> MTHGAVKTYGIRLRVWGDYACFTRPEMKVERVSYDVMPPSAARGILEAIHWKPAIRWIVDRIHVLRPIVFDNVRRNEVSSKIPKPNPATAMRDRKPLYFLVDDGSNRQQRAATLLRNVDYVIEAHFELTDKAGAEDNAGKHLDIFRRRARAGQSFQQPCLGCREFPASFELLEGDVPLSCYAGEKRDLGYMLLDIDFERDMTPLFFKAVMEDDVITPPSRTSPEVRA;>MTAIANRYEFVLLFDVENGNPNGDPDAGNMPRIDPETGHGLVTDVCLKRKIRNHVALTKEGAERFNIYIQEKAILNETHERAYTACDLKPEPKKLPKKVEDAKRVTDWMCTNFYDIRTFGAVMTTEVNCGQVRGPVQMAFARSVEPVVPQEVSITRMAVTTKAEAEKQQGDNRTMGRKHIVPYGLYVAHGFISAPLAEKTGFSDEDLTLFWDALVNMFEHDRSAARGLMSSRKLIVFKHQNRLGNAPAHKLFDLVKVSRAEGSSGPARSFADYAVTVGQAPEGVEVKEML[7x];> MILQALHGYYQRMSADPDAGMPPYGTSMENISFALVLDAKGTLRGIEDLREQEGKKLRPRKMLVPIAEKKGNGIKPNFLWENTSYILGVDAKGKQERTDKCHAAFIAHIKAYCDTADQDLAAVLQFLEHGEKDLSAFPVSEEVIGSNIVFRIEGEPGFVHERPAARQAWANCLNRREQGLCGQCLITGERQKPIAQLHPSIKGGRDGVRGAQAVASIVSFNNTAFESYGKEQSINAPVSQEAAFSYVTALNYLLNPSNRQKVTIADATVVFWAERSSPAEDIFAGMFDPPSTTAKPESSNGTPPEDSEEGSQPDTARDDPHAAARMHDLLVAIRSGKRATDIMPDMDESVRFHVLGLSPNAARLSVRFWEVDTVGHMLDKVGRHYRELEIIPQFNNEQEFPSLSTLLRQTAVLNKTENISPVLAGGLFRAMLTGGPYPQSLLPAVLGRIRAEHARPEDKSRYRLEVVTYYRAALIKAYLIRNRKLEVPVSLDPARTDRPYLLGRLFAVLEKAQEDAVPGANATIKDRYLASASANPGQVFHMLLKNASNHTAKLRKDPERKGSAIHYEIMMQEIIDNISDFPVTMSSDEQGLFMIGYYHQRKALFTKKNKEN;>VSLDPARTDRPYLLGRLFAVLEKAQEDA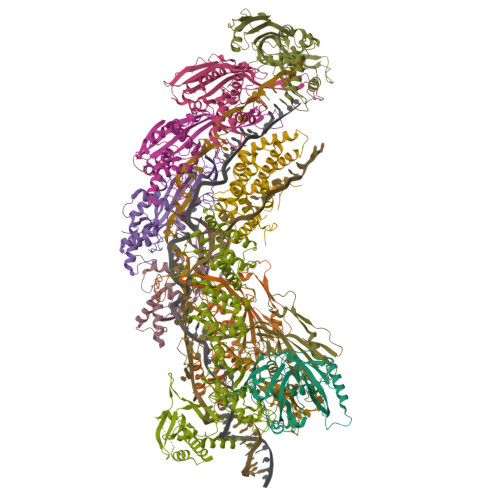VPGANATIKDRYLASASANPGQVFHMLLKNASNHTAKLRKDPERKGSAIHYEIMMQEIIDNISDFPVTMSSDEQGLFMIGYYHQRKALFTKKNKEN[2x]>EWQENKSWNAHFTEHKSQGVVVLWNENKQQGFTNNLKRANQAFLPASTFKIPNSLIALDLGVVKDEHQVFKWDGQTRDIATWNRDHNLITAMKYSVVPVYQEFARQIGEARMSKMLHAFDYGNEDISGNVDSFWLDGGI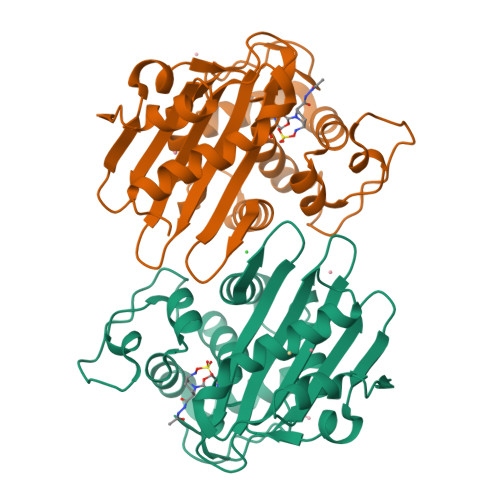RISATEQISFLRKLYHNKLHVSERSQRIVKQAMLTEANGDYIIRAKTGYSTRIEPKIGWWVGWVELDDNVWFFAMNMDMPTSDGLGLRQAITKEVLKQEKIIP[2x]> SSTLTPMHLRKAKLMFFWVRYPSSAVLKMYFPDIKFNKNNTAQLVKWFSNFREFYYIQMEKYARQAVTEGIKTPDDLLIAGDSELYRVLNLHYNRNNHIEVPQNFRF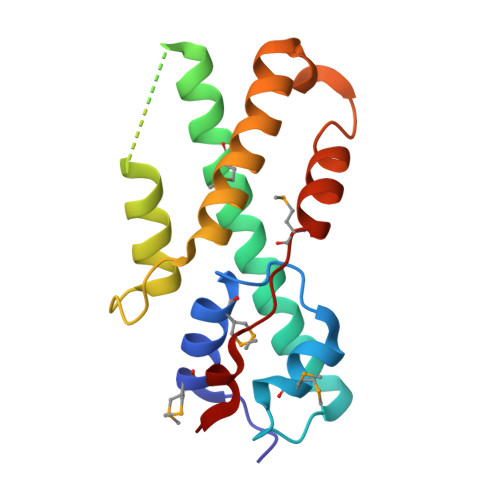VVESTLREFFRAIQGGKDTEQSWKKSIYKIISRMDDPVPEYFKSP>GSASLTEIEHLVQSVCKSYRETCQLRLEDLLRQRSNIFSREEVTGYQRKSMWEMWERCAHHLTEAIQYVVEFAKRLSGFMELCQNDQIVLLKAGAMEVVLVRMCRAYNADNRTVFFEGKYGGMELFRALGCSELISSIFDFSHSL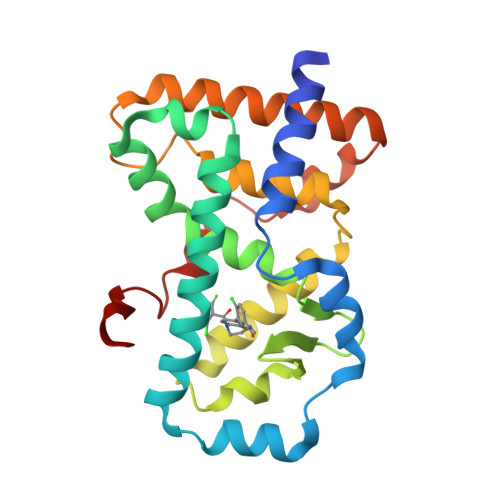SALHFSEDEIALYTALVLINAHRPGLQEKRKVEQLQYNLELAFHHHLCKTHRQSILAKLPPKGKLRSLCSQHVERLQIFQ[2x]>[2x]MSQVGGRGDRCTQEVQGLVHGAGDLSASLAENSPTMSQNGYFEDSSYYKCDTDDTFEAREEILGDEAFDTANSSIVSGESIRFFVNVNLEMQATNTENEATSGGCVLLHTSRKYLKLKNFKEEIRAHRDLDGFLAQASIVLNETATSLDNVLRTMLRRFARDPDNNEPNCNLDLLMAMLFTDAGAPMRGKVHLLSDTIQGVTATVTGVRYQQSWLCIICTMKALQKRHVCISRLVRPQNWGENSCEVRFVILVLAPPKMKSTKTAMEVARTFATMFSDIAFRQKLLETRTEEEFKEALVHQRQLLTMVSHGPVAPRTKERSTVSLPAHRHPEPPKCKDFVPFGKGIREDIARRFPLYPLDFTDGIIGKNKAVGKYITTTLFLYFACLLPTIAFGSLNDENTDGAIDVQKTIAGQSIGGLLYALFSGQPLVILLTTAPLALYIQVIRVICDDYDLDFNSFYAWTGLWNSF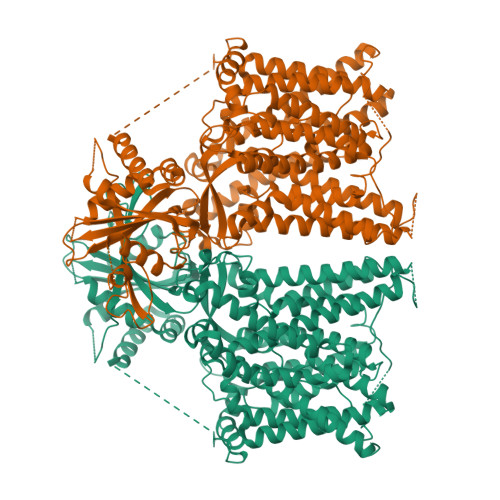FLALYAFFNLSLVMSLFKRSTEEIIALFISITFVLDAVKGTVKIFWKYYYGHYLDDYHTKRTSSLVSLSGLGASLNASLHTALNASFLASPTELPSATHSGQATAVLSLLIMLGTLWLGYTLYQFKKSPYLHPCVREILSDCALPIAVLAFSLISSHGFREIEMSKFRYNPSESPFAMAQIQSLSLRAVSGAMGLGFLLSMLFFIEQNLVAALVNAPENRLVKGTAYHWDLLLLAIINTGLSLFGLPWIHAAYPHSPLHVRALALVEERVENGHIYDTIVNVKETRLTSLGASVLVGLSLLLLPVPLQWIPKPVLYGLFLYIALTSLDGNQLVQRVALLLKEQTAYPPTHYIRRVPQRKIHYFTGLQVLQLLLLCAFGMSSLPYMKMIFPLIMIAMIPIRYILLPRIIEAKYLDVMDAEHRP(2S)-2-aminopent-4-enoic acid | C5 H9 N O2 | 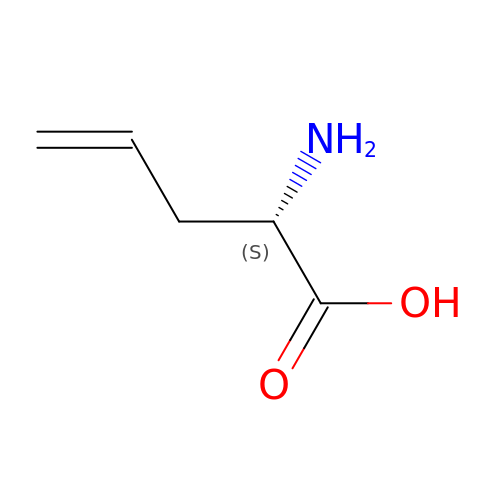WNNNWFKQCKFSDK-BYPYZUCNSA-N> MASLTVKAYLLGKEDAAREIARFSFSFSPEPEAEAEAAAGPGP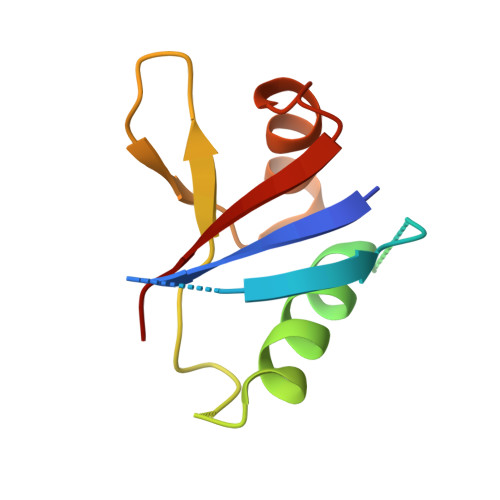CERLLSRVAALFPALRPGGFQAHYRDEDGDLVAFSSDEELTMAMSYVKDDIFRIYIKEK(2~{S})-2-[[(2~{S})-1,4-bis(oxidanyl)-1,4-bis(oxidanylidene)butan-2-yl]sulfamoylamino]pentanedioic acid | C9 H14 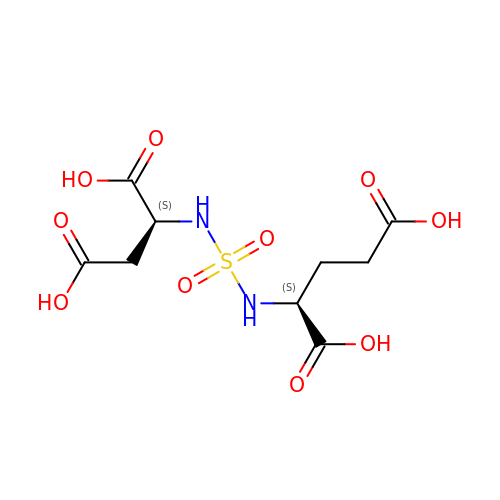N2 O10 S | YMLMAINCBMGBCN-WHFBIAKZSA-N> GPGSSHWTSKVHESVIGRNPEGQLGFELKGGAENGQFPYLGEVKPGKVAYESGSKLVSEELLLEVNETPVAGLTIRDVLAVIKHCKDPLRLKCVKQGGIVDKDLRHYLNLRFQKGSVDHELQQIIRDNLYLRTVPCTTRPHKEGEVPGVDYIFITVEEF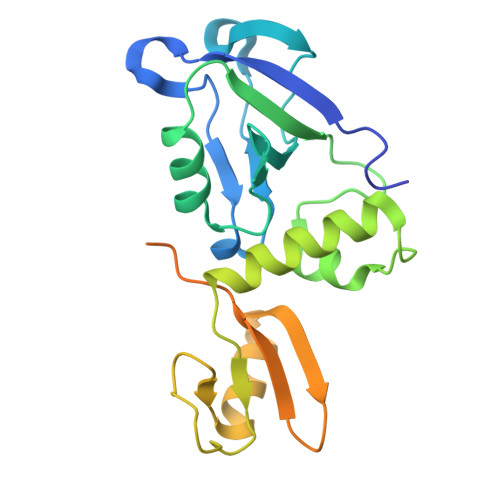MELEKSGALLESGTYEDNYYGTPKPPAEPAPLLNVTDQILPGATPSAEGKRKRNKSVTNMEKASIEPPEEEEEER> GSHMASPNGQTKPLPALKLALEYIVPAMNKHGICVVDDFLGKETGQQIGDEVRALHDTGKFTDGQLVSQKSDSSKDIRGDKITWIE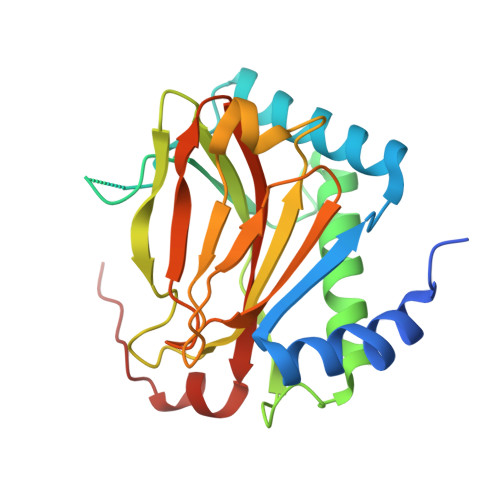GKEPGCETIGLLMSSMDDLIRHCNGKLGSYKINGRTKAMVACYPGNGTGYVRHVDNPNGDGRCVTCIYYLNKDWDAKVSGGILRIFPEGKAQFADIEPKFDRLLFFWSDRRNPHEVQPAYATRYAITVWYFDADERAAAKVKYLTGE>[2x]TDLKASSLRALKLMHLATSANDDDTDEKVIALCHQAKTPVGTTDAIFIYPRFIPIARKTLKEQGTPEIRICTSTNFPHGNDDIDIALAETRAAIAYGADSVAVVFPYRALMAGNEQVGFDLVKACKEACAAANVLLAVIIETGELKDEALIRKASEISIKAGADNIVTSTGKVAVGA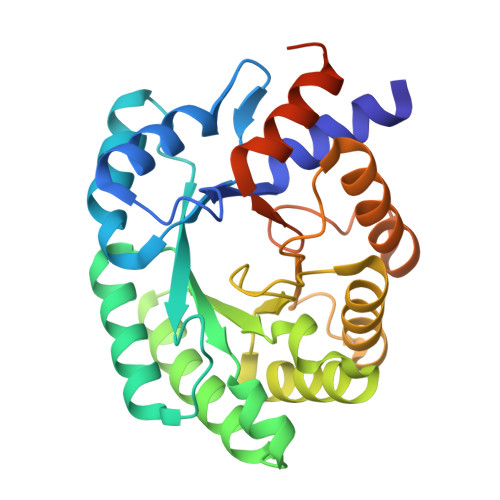TPESARIMMEVIRDMGVEKTVGFIPVGGVRTAEDAQKYLAIADELFGADWADARHYAFGASASLLASLLKALGHGDGKSASSYGSLEHHHHHH>MMIMLDPFSEKAKELLKGFGSINDFMDAIPKIVSVDDVIERIRVVKNEKLIDKFLDQDNVMDLAQFYALLGALSYSPYGIELELVKKANLIIYSERLKRKKEIKPEEISIDVSTAIEFPTEDVRKIERVYGKIPEYTMKISDFLDLVPDEKLANYYIYEGRVYLKREDLIRIWSKAFERNVERGVNMLYEIRDELPEFYRKVLGEIQAFAEEEFGRKFGE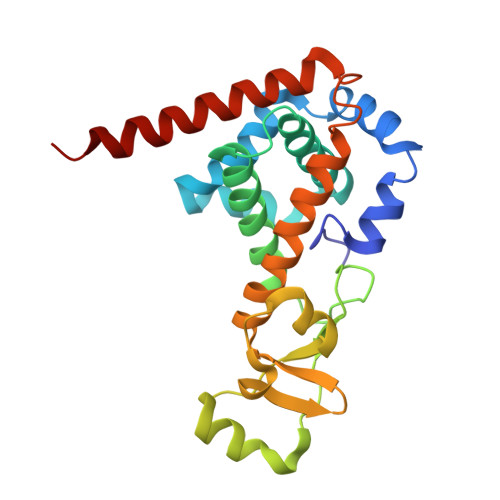IQ[3x]MIXED CARBAMIC PHOSPHORIC ACID ANHYDRIDE OF 7,8-DIAMINONONANIC ACID | 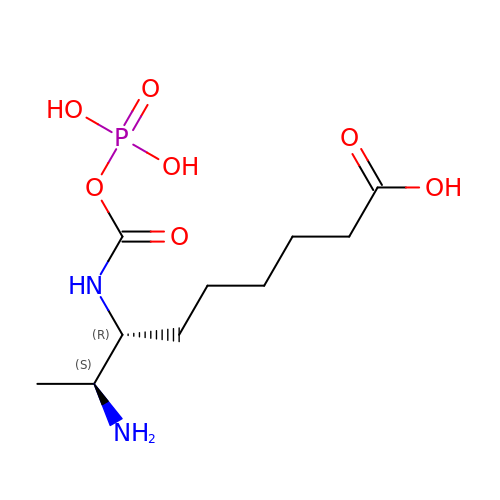C10 H21 N2 O7 P | UJJZZEABROBUCE-JGVFFNPUSA-N> SNAEKGLEIAQERKARDEGWGDSIATMEMILKNAQGESSTRLMRLKSLEVEGDGDKGLTIFDQPRDVTGTAFLNHSHTIGADDQWLYLPALKRVKRISSRNKSGPFMGSEFAYEDLSSFEIEKYRFNHLKDEKFNGQDVFVLEQIPTDKNSGYTKQVVWLDKAHYRPLKVEFYDRKGALLKTLTFANYKQYLDKYWRAHTMAMTNHQTGKSTELNT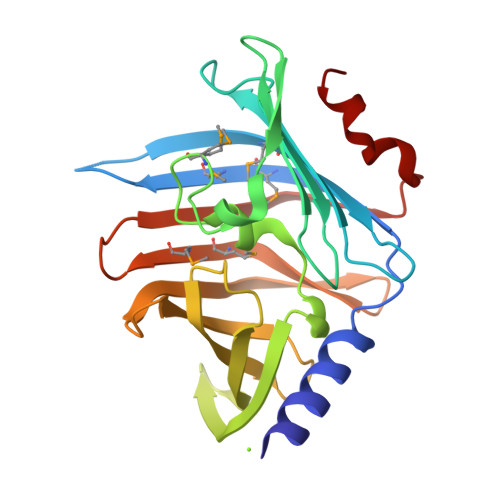SDLRFQTGLEENDFNKNVLKR> MLHSLRFLPMLTLLIVLPVIGALLMPLLPERVLRSVALVIAGLTFALSLWMLTQFDVHQSALQFTEFVPWLLPLGLNYSLGVDGLSLPLIVLGTFLTLGVVFTGEKTGQRLFYALVLLANAGITGALAAQNLLLFFLFYELELVPFYLLILIWGGQRREQAAVKFLIYTAVSGILVLAAFLAMGWLTHAPSFDSADIQIAGLAPTTQGILLLLLILGFGIKMPLVPLHSWLPDAYVEASTPTAILLGGALAKLGAYGLVRFALGYFPEAWAQFSGLLAIVAAVGIAYGALAAIAQKDIKRMVAYSSIGHMSYVLLAAAAHTHLSMVGAIAQMISHGLILALLFYLVGVIETKVGTRELNVLNGLLNPLRGLPTTSALLILGGMASAGIPGLVGFVAEFLIFQGSYGMFPLPTLVAVVGTGLTAVYFVIMINRTCFGRLDNRTAYYPRVVWSEKMPALVLTLLIVFLGVQPTWLVRWSETTSAQIVAAVPRTNEL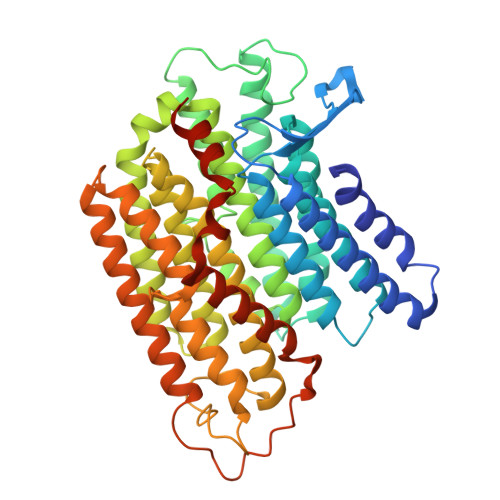VATLAKR Within the elongasome, the SEDS (shape, elongation, division, and sporulation) protein RodA catalyzes PG transglycosylation in concert with the PG cross-linking activity of PBP2, a class B penicillin-binding protein (bPBP). Here, we show that PBP2, which is the major enzyme responsible for bacterial cell shape and a target for the diazabicyclooctane (DBO) class of β-lactamase inhibitors, holds a noteworthy zinc-binding site in the transpeptidase domain. We found that Zn coordination is critical for the stability of PBP2 and for proper cell wall shape maintenance. The structure of PBP2 retains the typical bimodular fold of class bPBPs consisting of an elongated N-terminal module known as the pedestal domain and a C-terminal module bearing the TPase active site.

We generated an X-ray crystal structure of PBP2 at 2.65 Å resolution containing two macromolecules in the asymmetric unit. As the two protein chains were structurally similar (root mean square deviation of 1.8 Å for 511 matching Cα atoms), structure description will be focused on chain A based on model completeness. The pedestal domain of PBP2 (aa 53 to 243) is further organized into three subdomains known as anchor (aa 53 to 68 and 216 to 243), head (aa 78 to 165), and linker (aa 166 to 215). The TPase domain of PBP2 (aa 244 to 672) is mostly α-helical in nature (α8 to α19), and the catalytic site lies at the interface between an antiparallel five-β–stranded sheet (β10, β11, and β20 to β22) and the α-helical cluster (α10 to α17). The catalytic site of PBP2 encompasses strictly conserved residues in DD-TPases arranged in the following motifs: S(326)-x(T327)-x(I328)-K(329) containing the catalytic serine, S(383)-x(C384)-N/D(D385), and K(537)-T/S(T538)-G(539)-T(540). During the course of model building and refinement, we detected an extra region of electron density lying above the active site cleft and that was consistent with a metal coordination site, later assigned to zinc. Moreover, inductively coupled plasma mass spectrometry (ICP-MS) analysis of PBP2 in solution confirmed the binding of zinc to the protein at an equimolar ratio, therefore excluding the binding of zinc as a mere crystallization artifact. The Zn-binding site is enclosed on one side by the β12 to β15 hairpin region that extends over the top of the TPase domain. As a result, the zinc atom is shielded from solvent and sits atop the catalytic Ser326, from which is only 10.2 Å away (distance Zn–Ser326 Oγ). The zinc ion is tetrahedrally coordinated by the following residues: Asp350, located at the C terminus of β12, Asp365 and His371, positioned on a loop connecting β14 and β15, and Cys384, situated on a short loop connecting α11 and α12.

>[2x]MAHHHHHHSAALEVLFQGPGYQASDKNRIRLQPLPPARGYIYDRNGVLLADNYPVFTATLSKADVENVDTVIEQLQPILELTQEDVDRFKSRIKTARKTERVAIKLNLTETNIAKFSEVKYKFPGVRIETQMTRYYPHGDLFAHVIGYVGRINDKELKSIDKDLYAGTNLIGKIGVEKSYEDLLHGTPGYESVEADAHSNILRHLGRKDPTRGNDLYLSLDYGLQVVASQQLAGRRGAIVAIDPRTGEILALVSSPSFNPNLFVTGINHKDYSSLRDNIDQPLYNRAVQGVYPPGSTIKPMEAMGGLHYGIVDWATAISDPGYFHLPGDSHKFRDWKKTGHGIVNMHKAIIMSCDTYFYILANQMGIDQMNQWMRQFGFGQKTGVDLPSESEGLYPNPEWKMRTRKSKWMKGETISVSIGQGAFTATPLQLAMATAITANHGSHVVPHVLRATHGAKPFTVRNAPDGKINFNGTDEDWVKMREAMIDVIQSGTGRGIRTPLYQIAGKTGTAQVKSIAQGKRYNEAALSERQLDHGLFVGFAPADKPEIAIAVIWENGRHGGSAAQLAKPVFDYWLLTRKKNPIRPANHQVNGGLMTAGIKPGELPSGNESASSTPATSAPTSAAASTPQATPTRPATNEVDE>PSVYDAAAQLTADVKKDLRDSWKVIGSDKKGNGVALATTLFADNQETIGYFKRLGDVSQGMANDKLRGHSITLMYALQNFIDQLDNPDDLVCVVEKFAVNHITRKISAAEFGKINGPIKKVLASKNFGDKYANAWAKLVAVVQA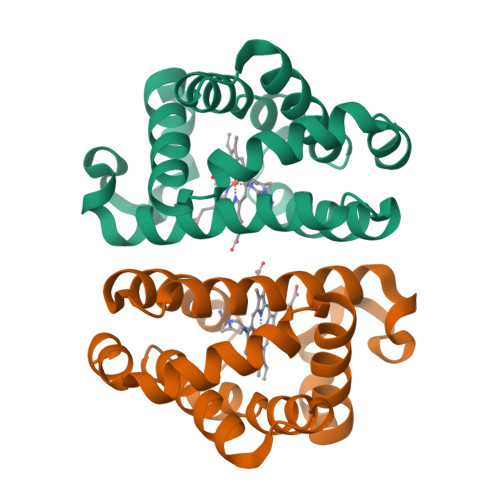AL[2x]>MGCTLSAEDKAAVERSKMIDRNLREDGERRAVRRLVKILLLGAGESGKSTFLKQMRIIHGREFDQKALLEFRDTIFDNILKGSRVLVDARDKLGIPWQHSENEKHGMFLMAFENKAGLPVEPATFQLYVPALSALWRDSGIREAFSRRSEFQLGESVKYFLDNLDRIGQLNYFPSKQDILLARKATKGIVEHDFVIKKIPFKMVDVGGQRSQRQKWFQCFDGITSILFMVSSSEYDQVLMEDRRTNRLVESMNIFETIVNNKLFFNVSIILFLNKMDLLVEKVKSVSIKKHFPDFKGDPHRLEDVQ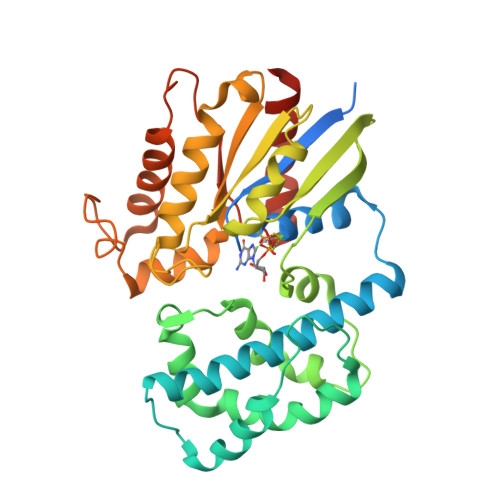RYLVQCFDRKRRNRSKPLFHHFTTAIDTENIRFVFHAVKDTILQENLKDIMLQ[2x]> MDETGKE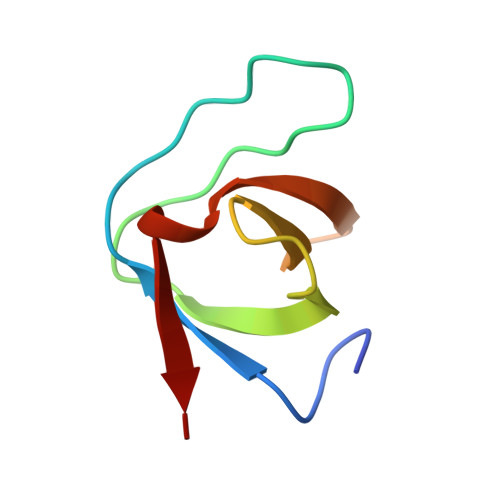LVLVLYDYQEKSPREVTIKKGDILTLLNSTNKDWWKIEVNDRQGFVPAAYLKKLD>[4x]MKTYHLNNDIIVTQEQLDHWNEQL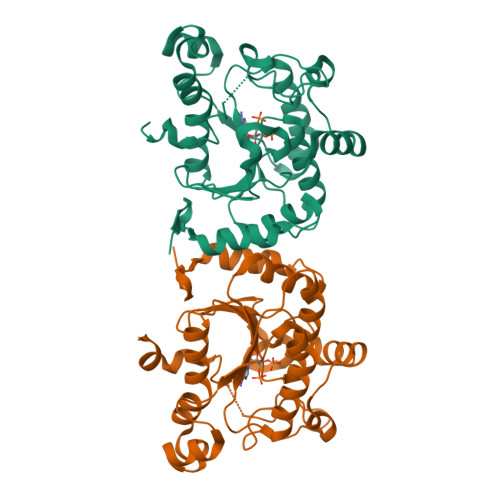IKLETPQEIIAWSIVTFPHLFQTTAFGLTGLVTIDMLSKLSEKYYMPELLFIDTLHHFPQTLTLKNEIEKKYYQPKNQTIHVYKPDGCESEADFASKYGDFLWEKDDDKYDYLAKVEPAHRAYKELHISAVFTGRRKSQGSARSQLSIIEIDELNGILKINPLINWTFEQVKQYIDANNVPYNELLDLGYRSIGDYHSTQPVKEGEDERAGRWKGKAKTECGIHEASRFAQFLKQDA> CRFETSELQASVMISTPLFTDSWSSCNTANCNGSIKIHDIAGITYVAIPAVSMIQLGNLVGLPVTGDVLFPGLSSDEPLPMVDAAILKLFLQLKIKEGLELELLGKKLVVITGHSTGGALAAFTALWLLSQSSPPSFRVFCITFGSPLLGNQSLSTSISRSRLAHNFCHVVSIHDLVPRSSNEQFWPFGTYLFCSDKGGVCLDNAGSVRLMFNILNTTATQNTEEHQRYGHYVFTLSHMFLKSRSFLGGSIPDNSYQAGVALAVEALGFSNDDTSGVLVKECIETATRIVRAPILRSAELANELASVLPARLEIQWYKDRCDASEEQLGYYDFFKRYSLKRDFKVNMSRIRLAKFWDTVIKMVETNELPFDFHLGKKWIYASQFYQLLAEPLDIANFYKNRDIKTGGHYLEGNRPKRYEVIDKWQKGVKVPEECVRSRYASTTQDTCFWAKLEQAKEWLDEARKESSDPQRRSLLREKIVPFESYANTLVTKKEVSLDVKAKNSSYSVWEANLKEFKCKMGYENEIEMVVDESDAMET;> MAFEALTGINGDLITRSWSASKQAYLTERYHKEEAGAVVIFAFQPSFSEKDFFDPDNKSSFGEIKLNRVQFPCMRKIGKGDVATVNEAFLKNLEAIIDPRTSFQASVEMAVRSRKQIVFTGHSSGGATAILATVWYLEKYFIRNPNVYLEPRCVTFGAPLVGDSIFSHALGREKWSRFFVNFVSRFDIVPRIMLARKASVEETLPHVLAQLDPRKSSVQESEQRITEFYTRVMRDTSTVANQAVCELTGSAEAFLETLSSFLELSPYRPAGTFVFSTEKRLVAVNNSDAILQMLFYTSQASDEQEWSLIPFRSIRDHHSYEELVQSMGKKLFNHLDGENSIESTLNDLGVSTRGRQYVQAALEEE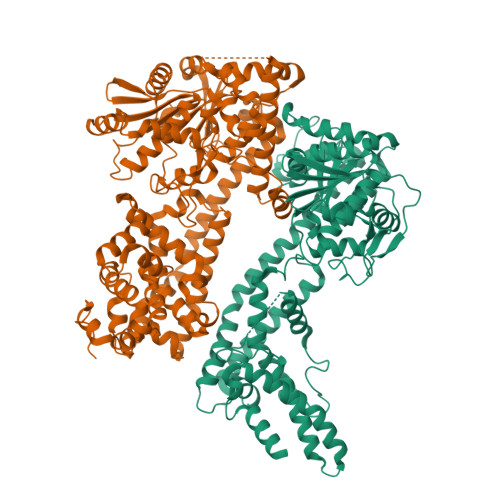KKRVENQKKIIQVIEQERFLKKLAWIEDEYKPKCQAHKNGYYDSFKVSNEENDFKANVKRAELAGVFDEVLGLMKKCQLPDEFEGDIDWIKLATRYRRLVEPLDIANYHRHLKNEDTGPYMKRGRPTRYIYAQRGYEHYILKPNGMIAEDVFWNKVNGLNLGLQLEEIQETLKNSGSECGSCFWAEVEELKGKPYEEVEVRVKTLEGMLGEWITDGEVDDKEIFLEGSTFRKWWITLPKNHKSHSPLRDYMMDEITDT> MSFITAFIWAYFLWLVLTAGSKGMLWSTQELIAGLIFASIVGYSTRNIIGEKASRFLNPVKWILFVAYAPVLFWGMVKANLDVAYRVITGKIRPGIVRVPVELENDAQYTILSNSITLTPGTLTVEACPEEKALYVHWINIPEGLEWPENSEPVSGPFEKWARRL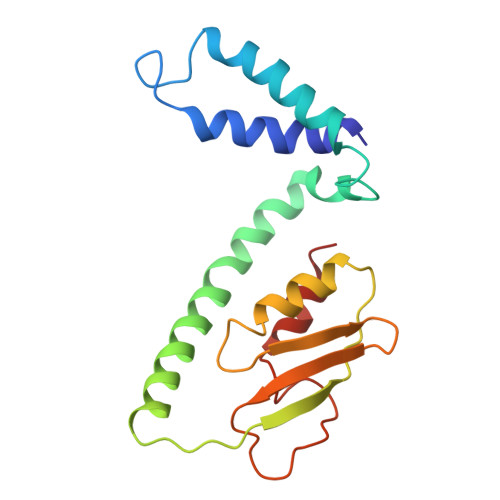GA>MHEEAVARAEAEKAKAELFSKAGVNQPPVYTQEMMERANSVMNEQGALVLNNTASSVQLAMTGTGVWTAAGDIAGNISKFFSNALEKVTIPEVSPLLMRISLGALWFHSEEAGAGSDIVPGRNLEAMFSLSAQMLAGQGVVIEPGATSVNLPVRGQLINSNGQLALDLLKTGNESIPAAVPVLNAVRDTATGLDKITLPAVVGAPSRTILVNPVPQPSVPTDTGNHQPVPVTPVHTGTEVKSVEMPVTTITPVSDVGGLRDFIYWRPDAAGTGVEAVYVMLNDPLDSGRF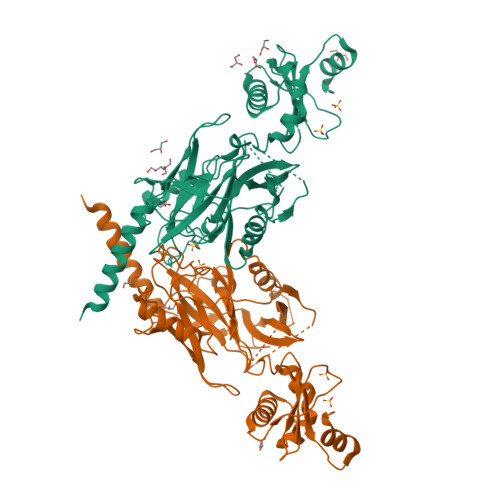SRKQLDKKYKHAGDFGISDTKKNRETLTKFRDAIEEHLSDKDTVEKGTYRREKGSKVYFNPNTMNVVIIKSNGEFLSGWKINPDADNGRIYLETGEL[2x]>VAFTEKQDALVSSSFEAFKANIPQYSVVFYTSILE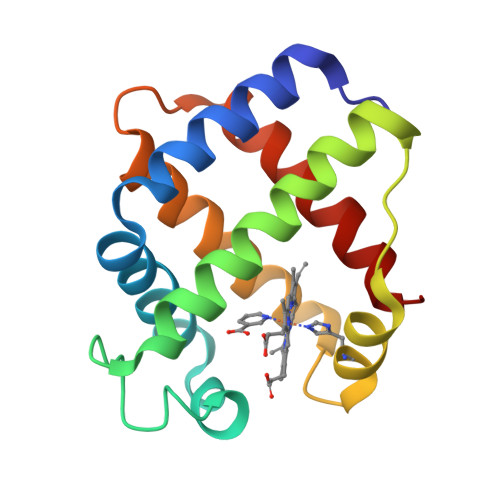KAPAAKDLFSFLANGVDPTNPKLTGHAEKLFALVRDSAGQLKASGTVVADAALGSVHAQKAVTDPQFVVVKEALLKTIKAAVGDKWSDELSRAWEVAYDELAAAIKKA[2x]>GAGAGAGAGAGMEQTYFISGANRGIGFSVVQRLAAKSGVKVIATARDPASATALNELAKENPQVKVVQLDISDEESIKKIAKNVSQYTDSI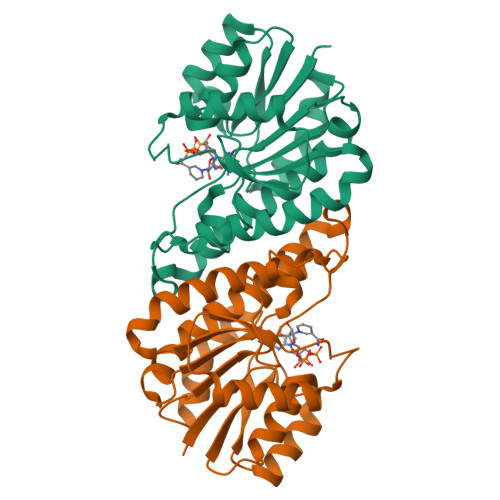DVFVSNAAIAKSFGPLLNTPREQWIEHFFTNVLGPIRLFQELYPLIKKGTQKKVFFISSNAGSLNLDFGLDFSAFGQSKAALNYSTKELARQLKPENFIVAAVHPGFVTTDMGKGGERAFTAVDEVSAKKFFTPETKITPEESAAALCKLFESLNTTGKYLSYDGTELPW[4x]>MAHHHHHHLVPRGSHETEQSVDLETVSVVGKSRPRATSGLLHTSTASDKIISGDTLRQKAVNLGDALDGVPGIHASQYGGGASAPVIRGQTGRRIKVLNHHGETGDMADFSPDHAIMVDTALSQQVEILRGPVTLLYSSGNVAGLVDVADGKIPEKMPENGVSGELGLRLSSGNLEKLTSGGINIGLGKNFVLHTEGLYRKSGDYAVPRYRNLKRLPDSHADSQTGSIGLSWVGEKGFIGVAYSDRRDQYGLPAHSHEYDDCHADIIWQKSLINKRYLQLYPHLLTEEDIDYDNPGLSCGFHDDDNAHAHTHSGRPWIDLRNKRYELRAEWKQPFPGFEALRVHLNRNDYRHDEKAGDAVENFFNNQTQNARIELRHQPIGRLKGSWGVQYLQQKSSALSAISEAVKQPMLLDNKVQHYSFFGVEQANWDNFTLEGGVRVEKQKASIQYDKALIDRENYYNHPLPDLGAHRQTARSFALSGNWYFTPQHKLSLTASHQERLPSTQELYAHGKHVATNTFEVGNKHLNKERSNNIELALGYEGDRWQYNLALYRNR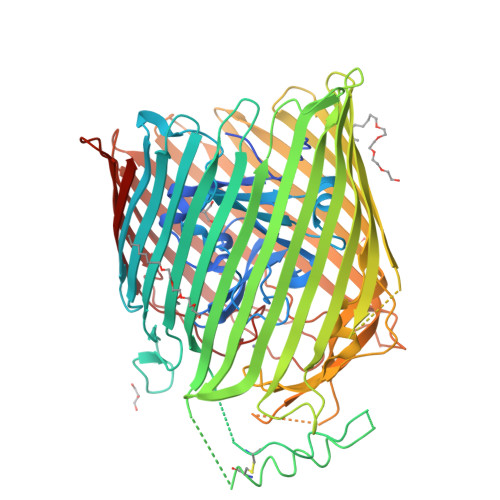FGNYIYAQTLNDGRGPKSIEDDSEMKLVRYNQSGADFYGAEGEIYFKPTPRYRIGVSGDYVRGRLKNLPSLPGREDAYGNRPFIAQDDQNAPRVPAARLGFHLKASLTDRIDANLDYYRVFAQNKLARYETRTPGHHMLNLGANYRRNTRYGEWNWYVKADNLLNQSVYAHSSFLSDTPQMGRSFTGGVNVKF[2x]HUPERZINE B | C16 H20 N2 O | 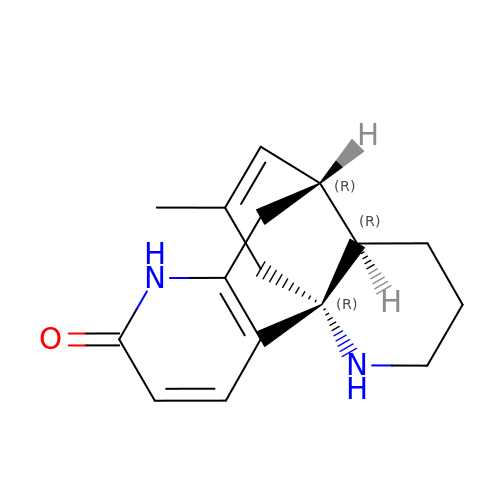YYWGABLTRMRUIT-HWWQOWPSSA-N>SNAMSSSSSPPHQLNHFSDVANKAANAAGDVIRKYFRKNNFDIIHKNDLSPVTIADQSAEEAMVSVILDNFPSHAVYGEEKGWRCKQDSADYVWVLDPIDGTKSFITGKPLFGTLIALLQNGTPILGIIDQPVLKERWIGITGKRTTLNGQEVSTRTCADLSQAYLYTTSPHLFSGDAEEAFIRVRDKVKIPLYGCDCYAYALLSSGFVDLVVESGLKPYDFLALIPVIEGSGGVITDWKGHQLRWEASPLSIATSFNVVA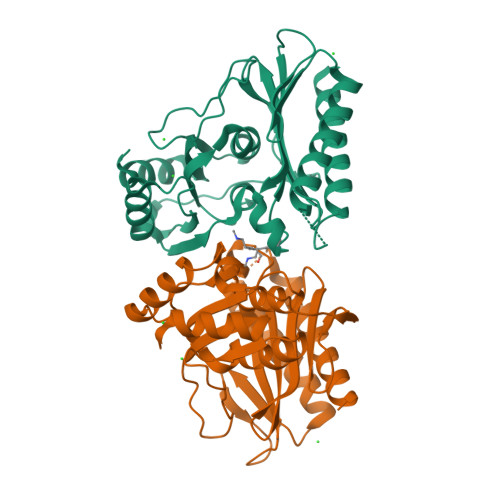AGDKQIHQQALDSLQW[4x]>[2x]MVLYFIGLGLYDERDITVKGLEIAKKCDYVFAEFYTSLMAGTTLGRIQKLIGKEIRVLSREDVELNFENIVLPLAKE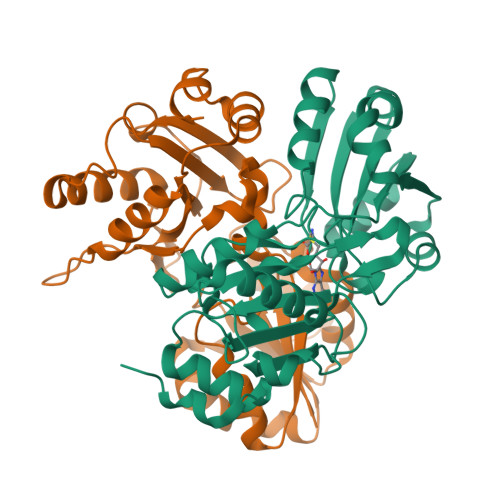NDVAFLTPGDPLVATTHAELRIRAKRAGVESYVIHAPSIYSAVGITGLHIYKFGKSATVAYPMGNWFPTSYYDVIKENAERGLHTLLFLDIKAEKRMYMTANEAMELLLKVEDMKKGGVFTDDTLVVVLARAGSLNPTIRAGYVKDLIREDFGDPPHILIVPGKLHIVEAEYLVEIAGAPREILRVNV> GAPATVTEQGEDITSKKDRGVLKIVKRVGNGEETPMIGDKVYVHYKGKLSNSKKFDSSHDRNEPFVFSLGKGQVIKAW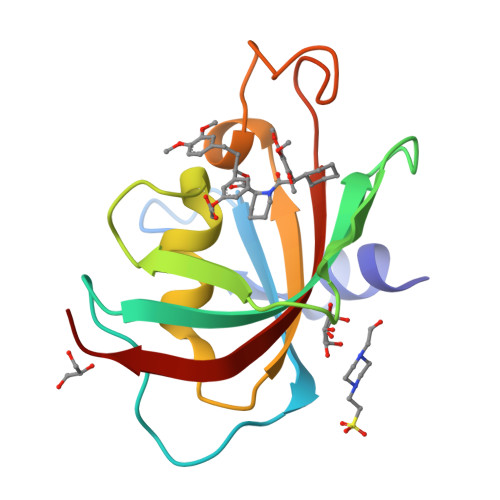DIGVATMKKGEIAHLLIKPEYAYGSAGSLPKIPSNATLFFEIELLDFKGE> KVEDFKEDKEKAKEWGKEKEKEWKLTATEKGKMNNFLDNKNDIKTNYKEITFSMAGSFEDEIKDLKEIDKMFDKTNLSNSIITYKNVEPTTIGFNKSLTEGNTINSDAMAQFKEQ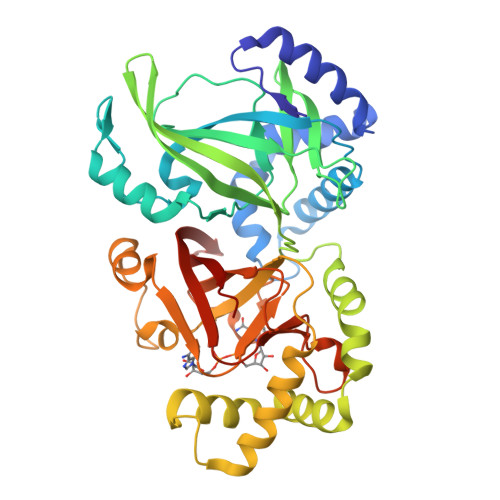FLDRDIKFDSYLDTHLTAQQVSSKERVILKVTVPSGKGSTTPTKAGVILNNSEYKMLIDNGYMVHVDKVSKVVKKGVECLQIEGTLKKSLDFKNDINAEAHSWGMKNYEEWAKDLTDSQREALDGYARQDYKEINNYLRNQGGSGNEKLDAQIKNISDALGKKPIPENITVYRWCGMPEFGYQISDPLPSLKDFEEQFLNTIKEDKGYMSTSLSSERLAAFGSRKIILRLQVPKGSTGAYLSAIGGFASEKEILLDKDSKYHIDKVTEVIIKGVKRYVVDATLLTN>[2x]GSHMKKHTGYVGLKNQGATCYMNSLLQTLFFTNQLRKAVYMMPTEGDD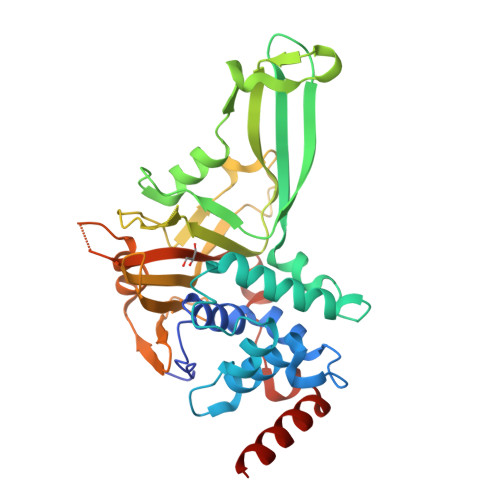SSKSVPLALQRVFYELQHSDKPVGTKKLTKSFGWETLDSFMQHDVQELCRKLLDNVENKMKGTCVEGTIPKLFRGKMVSYIQCKEVDYRSDRREDYYDIQLSIKGKKNIFESFVDYVAVEQLDGDNKYDAGEHGLQEAEKGVKFLTLPPVLHLQLMRFMYDPQTDQNIKINDRFEFPEQLPLDEFLQKTDPKDPANYILHAVLVHSGDNHGGHYVVYLNPKGDGKWCKFDDDVVSRCTKEEAIEHNYGGHDDDLSVRHCTNAYMLVYIRESKLSEVLQAVTDHDIPQQLVERLQEEKRIEAQK4-{3-[(4-chlorophenyl)amino]-3-oxopropyl}-3-({[5-(propan-2-yl)-4,5,6,7-tetrahydro[1,3]thiazolo[5,4-c]pyridin-2-yl]carbonyl}amino)benzoic 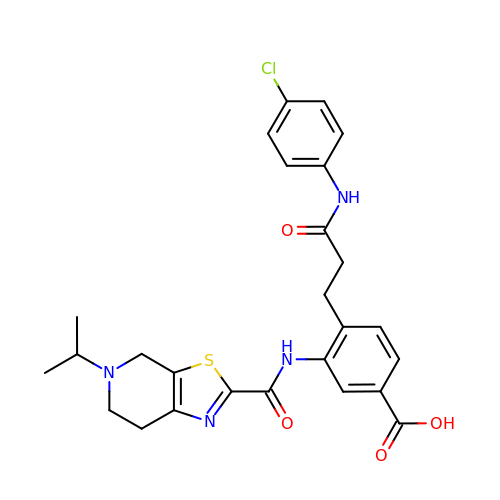acid | C26 H27 Cl N4 O4 S | FQNIFNHOEQFSHE-UHFFFAOYSA-N> MAVKKIAIFGATGRTGLTTLAQAVQAGYEVTVLVRDSSRLPSEGPRPAHVVVGDVLQAADVDKTVAGQDAVIVLLGTRNDLSPTTVMSEGARNIVAAMKAHGVDKVVACTSAFLLWDPTKVPPRLQAV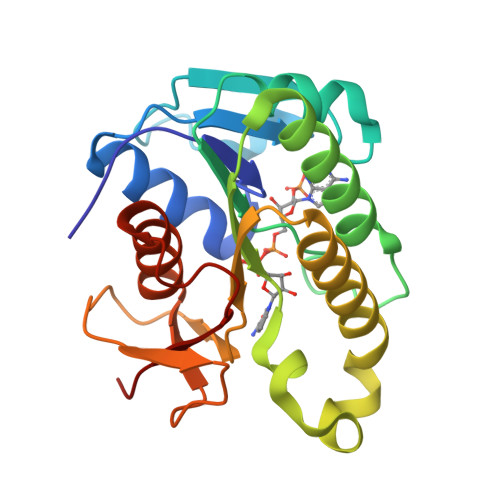TDDHIRMHKVLRESGLKYVAVMPPHIGDQPLTGAYTVTLDGRGPSRVISKHDLGHFMLRCLTTDEYDGHSTYPSHQY> MSQITIQARLISFESNRQQLWKLMADLNTPLINELLCQLGQHPDFEKWQQKGKLPSTVVSQLCQPLKTDPRFAGQPSRLYMSAIHIVDYIYKSWLAIQKRLQQQLDGKTRWLEMLNSDAELVELSGDTLEAIRVKAAEILAIAMPASESDSASPKGKKGKKEKKPSSSSPKRSLSKTLFDAYQETEDIKSRSAISYLLKNGCKLTDKEEDSEKFAKRRRQVEIQIQRLTEKLISRMPKGRDLTNAKWLETLLTATTTVAEDNAQAKRWQDILLTRSSSLPFPLVFETNE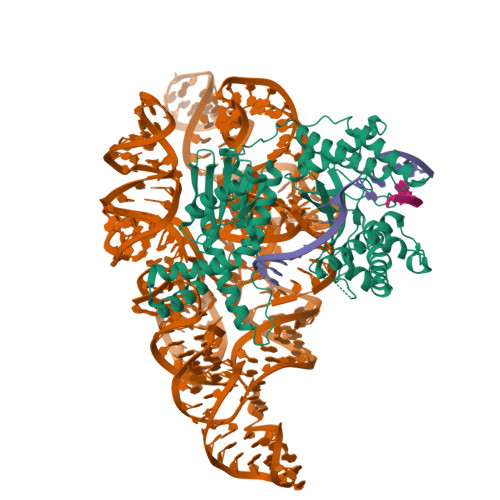DMVWSKNQKGRLCVHFNGLSDLIFEVYCGNRQLHWFQRFLEDQQTKRKSKNQHSSGLFTLRNGHLVWLEGEGKGEPWNLHHLTLYCCVDNRLWTEEGTEIVRQEKADEITKFITNMKKKSDLSDTQQALIQRKQSTLTRINNSFERPSQPLYQGQSHILVGVSLGLEKPATVAVVDAIANKVLAYRSIKQLLGDNYELLNRQRRQQQYLSHERHKAQKNFSPNQFGASELGQHIDRLLAKAIVALARTYKAGSIVLPKLGDMREVVQSEIQAIAEQKFPGYIEGQQKYAKQYRVNVHRWSYGRLIQSIQSKAAQTGIVIEEGKQPIRGSPHDKAKELALSAYNLRLTRRSGSEFELENLYFQ> MGSDKIHHHHHHENLYFQGMSTEQLLVLIAQNDIKDDIVDTLIELEFLSGFSLGNICGFSREHSHFNIKEQVEGYREFCKFEIMHPAAQQAALLTALALVCKHNPCRYWIMPIY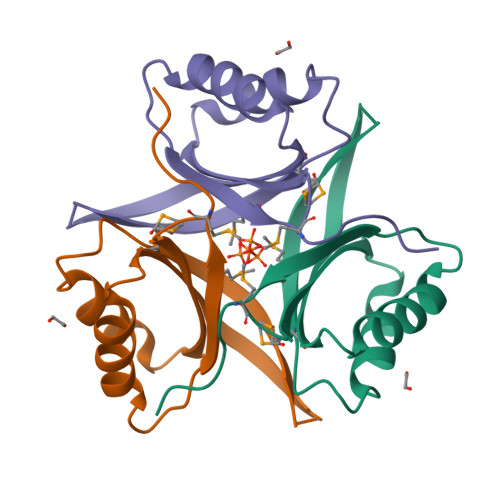QNGTLS>[2x]MYTEVRELVNFVCRYLFGHIPRRPVGIFGAELG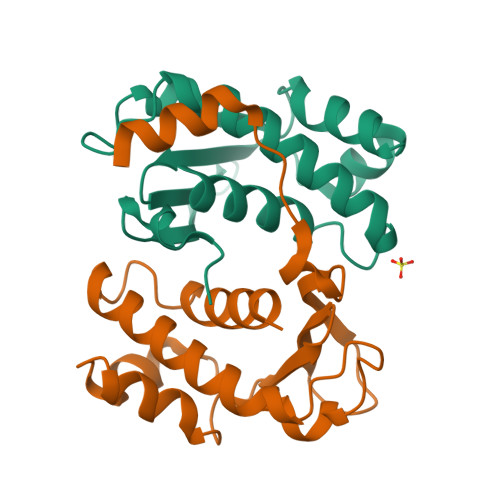NYLVSHFSSTWDVNHPKNGEMKRMINTTTSLCFASSAEEAGVPPSDVLRLLPTNMIIFANPGHVFVRLSENGIETPIWIGDVNADENYQSVPEYVVRTAAIRAEHHHHHH One of these highly populated repetitive folds is the αα-solenoid (SCOP a.118), whose most widespread superfamily is the tetratricopeptide repeat (TPR; a.118.8). The ﬁrst crystal structure of a TPR domain showed that the repeat units are helical hairpins, stacked into a continuous, right-handed superhelical architecture with an inner groove that mediates the interaction with target proteins. Here we show that such hairpins are detectable and that one of them, from the ribosomal protein RPS20, can be customized to yield a TPR fold by repetition, with only a small number of point mutations that are neutral for the parent organism. We concatenated three copies of RPS20-hhta as an initial construct, connected by the TPR consensus loop sequence (DPNN).

M4NΔC is M4N without stop helix. We conclude that in the amplified constructs, the observed interactions are more favorable than the interaction with the native stop helix, releasing it and rendering it prone to degradation. This led us to ask whether this helix is in fact dispensable. Indeed, an M4NΔC construct, which terminates with the B3 helix, showed the same stability and dimerization as M4N. We obtained two structures for M4NΔC from different crystal forms at 2.0 Å and 1.7 Å resolution, respectively, the first (CF I) with two dimers in the ASU and the second (CF II) with a single chain in the ASU, for which we constructed the dimer by crystallographic symmetry. (a) Two dimers in the ASU of M4NΔC CF I. (b) Dimer constructed by applying the crystallographic symmetry to the single chain in the ASU of M4NΔC CF II. All three dimers superimpose to the M4N dimer with Cα RMSD below 1.9 Å.

> MGNSIKTLSNLANLLAQEGKAEEAIKYMRKAVSLDPNNIKTLSNLANLLAQEGKAEEAIKYMRKAVSLDPNNIKTLSNLAVLLAQEGKAEEAIKYMRKAVSLIDKAAKG>[6x]IVRPPFTYATLIRQAIMESSDRQLTLNEIYSWFTRTFAYFRRNAATWKNAVRH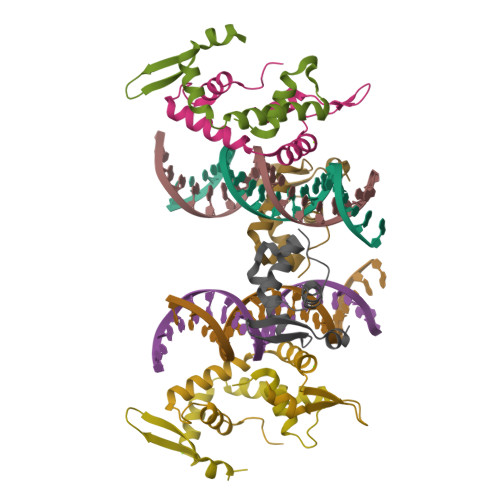NLSLHKCFVRVENVKGAVWTVDEVEYQKRRSQKITGSPTL>[12x]MSKSDVFHLGLTKNDLQGATLAIVPGDPDRVEKIAALMDKPVKLASHREFTTWRAELDGKPVIVCSTGIGGPSTSIAVEELAQLGIRTFLRIGTTGAIQPHINVGDVLVTTASVRLDGASLHFAPLEFPAVADFECTTALVEAAKSIGATTHV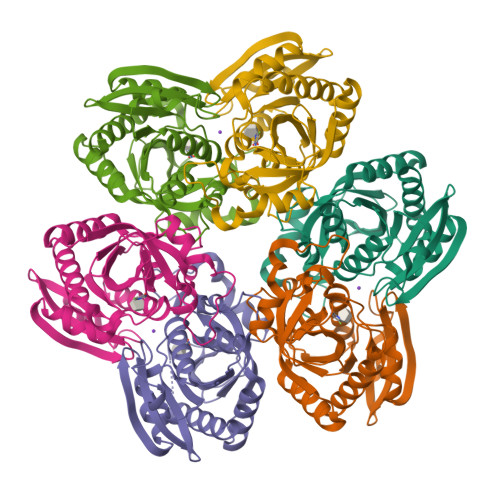GVTASSDTFYPGQERYDTYSGRVVRHFKGSMEEWQAMGVMNYEMESATLLTMCASQGLRAGMVAGVIVNRTQQEIPNAETMKQTESHAVKIVVEAARRLL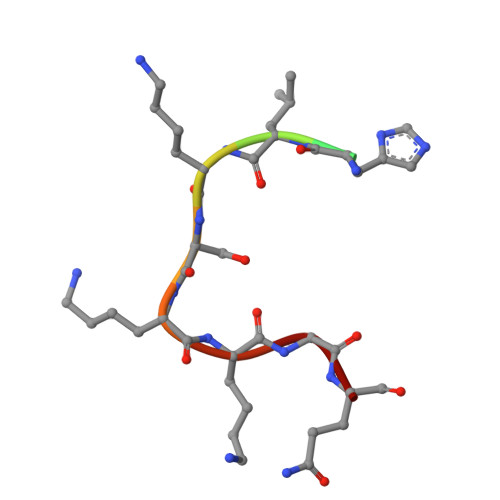> HSSHLKSKKGQ> QECTKFKVSSCRECIESGPGCTWCQKLNFTGPGDPDSIRCDTRPQLLMRGCAADDIMDPTSLAETQEDHNGGQKQLSPQKVTLYLRPGQAAAFNVTFRRAKLSSRVFLDHNALPDTLKVTYDSFCSNGVTHRNQPRGDCDGVQINVPITFQVKVTATECIQEQSFVI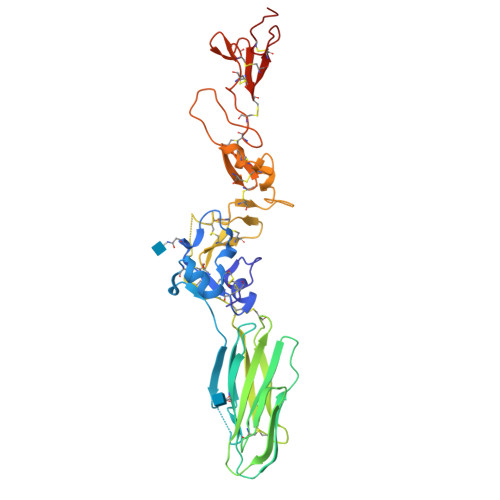RALGFTDIVTVQVLPQCECRCRDQSRDRSLCHGKGFLECGICRCDTGYIGKNCECQTQGRSSQELEGSCRKDNNSIICSGLGDCVCGQCLCHTSDVPGKLIYGQYCECDTINCERYNGQVCGGPGRGLCFCGKCRCHPGFEGSACQHHHH>SKTKPFSLPILTL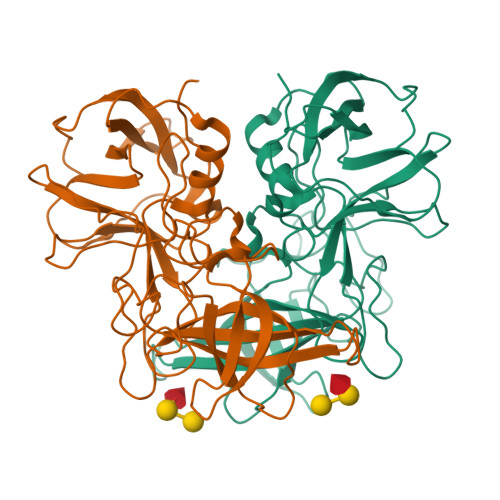SELTNSRFPVPIDSLFTAQNNVLQVQCQNGRCTLDGELQGTTQLLPSGICAFRGRVTAQINQRDRWHMQLQNLNGTTYDPTDDVPAPLGTPDFKGVVFGMVSQRNVGNDAPGSTRAQQAWVSTYSPQFVPKLGSVNLRISDNDDFQFQPTKFTPVGVNDDDDGHPFRQWELPNYSGELTLNMNLAPPVAPNFPGEQLLFFRSFVPCSGGYNQGIIDCLIPQEWIQHFYQESAPSQSDVALIRYVNPDTGRTLFEAKLHRSGYITVAHSGDYPLVVPANGHFRFDSWVNQFYSLAPM[2x]>[2x]GLEEEARELAEEAREVRRRAEELRRRAEEARETGEASEEHAAALLAEAAVLELKAVLLELEARRLLKESGGEVAREALELAREARREAREALEAAEEASE

We set out to design proteins that can switch between two well-defined and fully structured conformations. We reasoned that these goals could be collectively achieved with a “hinge”-like design in which two rigid domains move relative to each other while remaining individually folded. The hinge amplifies small local structural and chemical changes to achieve large global changes while the chemical environment for most residues remains similar throughout the conformational change, avoiding the need for global unfolding. Designing one of the resulting conformations to bind to a target effector couples the conformational equilibrium with target binding.

To explore whether peptide-responsive hinges could be turned into protein-responsive hinges, we used inpainting with RoseTTAFold to add two additional helices to a validated effector peptide, resulting in fully structured 3-helix bundles (3hb). For nine of our validated hinges we designed and experimentally characterized these effector proteins using SEC. Hinge-3hb binding was tested qualitatively by SEC and, for hinges which had a corresponding FRET construct, quantitatively with the FRET-labeled variant, and DEER was used in addition to FRET to confirm that 3hb binding caused the same conformational change as effector peptide binding. For two designs, 3hb05 and 3hb12, we obtained crystal structures that agreed well with the design models, indicating that the three-helix bundles are fully structured in isolation. The 3hb approach was able to rescue designs for which the peptide alone or the hinge-peptide complex had shown the tendency to form higher-order oligomers.>MAVPETRPNHTIYINNLNEKIKKDELKKSLHAIFSRFGQILDILVSRSLKMRGQAFVIFKEVSSATNALRSM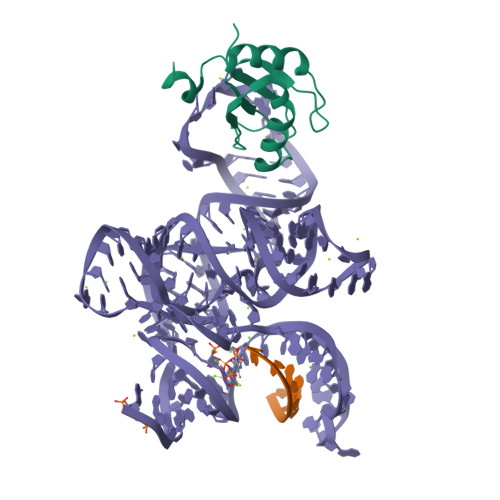QGFPFYDKPMRIQYAKTDSDIIAKMK[2x]> GSMSRSKRDNNFYSVEIGDSTFTVLKRYQNLKPIGSGAQGIVCAAYDAILERNVAIKKLSRPFQNQTHAKRAYRELVLMKCVNHKNIIGLLNVFTPQKSLEEFQDVYIVMELMDANLCQVIQMELDHERMSYLLYQMLCGIKHLHSAGIIHRDLKPSNIVVKSDCTLKILDFGLARTAGTSFMMTPYVVTRYYRAPEVILGMGYKENVDIWSVGCIMGEMIKGGVLFPGTDHIDQWNKVIEQLGTPCPEFMKKLQPTVRTYVENRPKYAGYSFEKLFPDVLFPADSEHNKLKASQARDLLSKM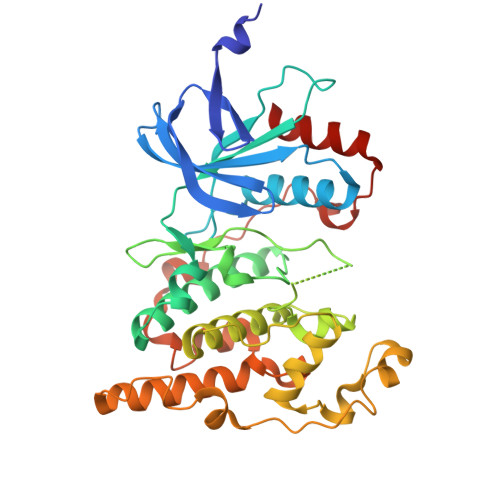LVIDASKRISVDEALQHPYINVWYDPSEAEAPPPKIPDKQLDEREHTIEEWKELIYKEVMDLE> GSEFPLDTSLRLKTFSSKSEYQLVVNAVRKLQESGFYWSAVTGGEANLLLSAEPAGTFLIRDSSDQRHFFTLSVKTQSGTKNLRIQCEGGSFSLQSDPRSTQPVPRFDCVLKLVHHYMPPQALPGSTPKRAYYIYSGGEKIPLV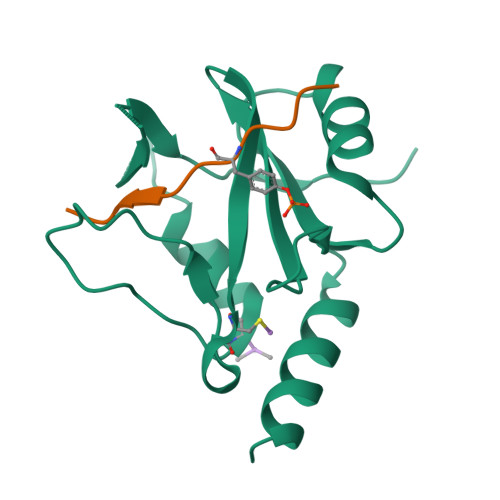LSRPLSSN;> STVEYSTVVHS> MPGPLGLLCFLALGLLGSAGPSGAAPPLCAAPCSCDGDRRVDCSGKGLTAVPEGLSAFTQALDISMNNITQLPEDAFKNFPFLEELQLAGNDLSFIHPKALSGLKELKVLTLQNNQLKTVPSEAIRGLSALQSLRLDANHITSVPEDSFEGLVQLRHLWLDDNSLTEVPVHPLSNLPTLQALTLALNKISSIPDFAFTNLSSLVVLHLHNNKIRSLSQHCFDGLDNLETLDLNYNNLGEFPQAIKALPSLKELGFHSNSISVIPDGAFDGNPLLRTIHLYDNPLSFVGNSAFHNLSDLHSLVIRGASMVQQFPNLTGTVHLESLTLTGTKISSIPNNLCQEQKMLRTLDLSYNNIRDLPSFNGCHALEEISLQRNQIYQIKEGTFQGLISLRILDLSRNLIHEIHSRAFATLGPITNLDVSFNELTSFPTEGLNGLNQLKLVGNFKLKEALAAKDFVNLRSLSVPYAYQCCAFWGCDSYANLNTEDNSLQDHSVAQEKGTADAANVTSTLENEEHSQIIIHCTPSTGAFKPCEYLLGSWMIRLTVWFIFLVALFFNLLVILTTFASCTSLPSSKLFIGLISVSNLFMGIYTGILTFLDAVSWGRFAEFGIWWETGSGCKVAGFLAVFSSESAIFLLMLATVERSLSAKDIMKNGKSNHLKQFRVAALLAFLGATVAGCFPLFHRGEYSASPLCLPFPTGETPSLGFTVTLVLLNSLAFLLMAVIYTKLYCNLEKEDLSENSQSSMIKHVAWLIFTNCIFFCPVAFFSFAPLITAISISPEIMKSVTLIFFPLPACLNPVLYVFFNPKFKEDWKLLKRRVTKKENLYFQGDYKDDDDKHHHHHHHH;> MQFRLFSFALIILNCMDYSHCQGNRWRRSKRASYVSNPICKGCLSCSKDNGCSRCQQKLFFFLRREGMRQYGECLHSCPSGYYGHRAPDMNRCARCRIENCDSCFSKDFCTKCKVGFYLHRGRCFDECPDGFAPLEETMECVEENLYFQGHHHHHHHHHH

Leucine-rich repeat-containing G protein-coupled receptor 4 (LGR4) plays a critical role in regulating the wingless-related integration site (Wnt) signaling pathway and is essential for organ development and carcinogenesis. LGR4, along with its ligand R-spondin (RSPO), potentiates Wnt/β-catenin signaling by recruiting its signaling suppressor, E3 ligase Zinc and Ring Finger 3 (ZNRF3), and inducing its membrane clearance. Cell surface-expressed LGR4/5, members of the class A G-protein coupled receptors (GPCR) family, have an extracellular domain (ECD) comprising 17 leucine-rich repeats (LRRs), followed by a seven-transmembrane domain (TMD), and an intracellular domain (ICD). ZNRF3/RNF43, LGR4, and RSPO form a ternary complex on the cell surface, which relieves ZNRF3/RNF43-mediated suppression of Wnt/β-catenin signaling and thereby potentiates pathway activation.

We purified the binary complex of human LGR4 and RSPO2 using gel-filtration chromatography from a mixture of individually purified LGR4 and RSPO2 (residues 20-143, Fu1-2 domains). We determined its structure using cryo-EM at an overall resolution of 4.0 Å. RSPO2 Fu1-2 domains exhibited an elongated form comprising multiple β-hairpins stabilized by disulfide bonds. RSPO2-bound LGR4 structure is almost identical to the apo LGR4 structure with an overall RMSD of 0.40 Å, indicating that RSPO2 binding does not induce any conformational differences in the LGR4 structure. This is in sharp contrast to the ‘push-pull’ activation mechanism of related LGR1-3, in which hormone bound to the receptor sterically clashes with the membrane, causing an upward movement of the ECD to avoid the clash, resulting in receptor activation. Upon RSPO2 binding, LGR4 undergoes no significant conformational changes in its transmembrane and extracellular domain structures or their relative orientations.>TELEHWPAPAARQLNALIEANANKGAYAVFDMDNTSYRYDLEESLLPYLEMKGVLTRDRLDPSLKLIPFKDQAGHKESLFSYYYRLCEIDDMVCYPWVAQVFSGFTLRELKGYVDELMAYGKPIPATYYDGDKLATLDVEPPRVFSGQRELYNKLMENGIEVYVISAAHEELVRMVAADPRYGYNAKPENVIGVTTLLKNRKTGELTTARKQIAEGKYDPKANLDLEVTPYLWTPATWMAGKQAAILTYIDRWKRPILVAGDTPDSDG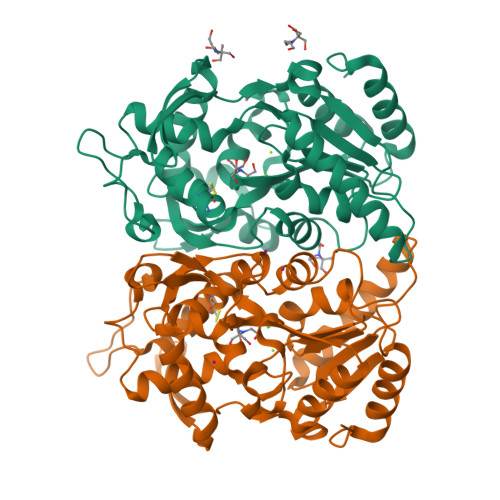YMLFNGTAENGVHLWVNRKAKYMEQINGMIKQHSAAQAKAGLPVTADRNWVIVTPEQIQ[4x]>AGHMYNPRCKDLDRDYFPSYHTTRFQDQPEPNLAVLEHFVRVTKQHGRELTEKQGITVDHLRYGEGRQLVDVFYSEKTTNQAPLFVFVHGGYWQEMDMSMSCSIVGPLVRRGYRVAVMDYNLCPQVTLEQLMTQFTHFLNWIFDYTEMTKVSSLTFAGH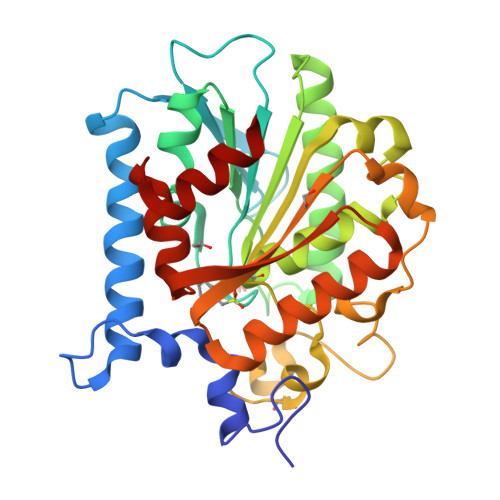SAGAHLLAQILMRPNVITAQRSKMVWALIFLCGVYDLRELSNLESVNPKNILGLNERNIESVSPMLWEYTDVTVWNSTKIYVVAAEHDSTTFIEQSRHYADVLRKKGYKASFTLFKGYDHFDIIEETAIDDSDVSRFLRNIEIE[2x]>MGDKPIWEQIGSSFINHYYQLFDNDRTQLGAIYIDASCLTWEGQQFQGKAAIVEKLSSLPFQKIQHSITAQDHQPTPDSC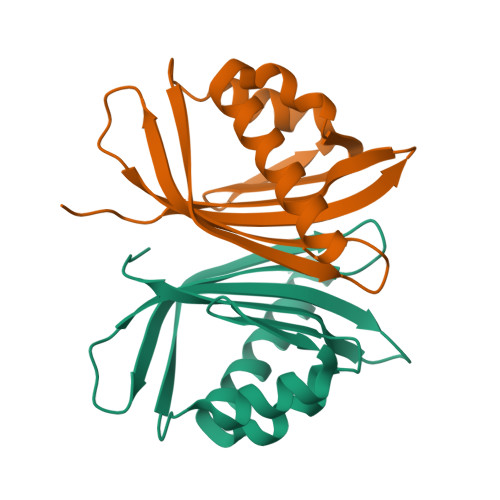IISMVVGQLKADEDPIMGFHQEFLLKNINDAWVCTNDMFRLALHNFG[2x]> GDVVEAVENAVARVADTIGSGPSNSQAVPALTAVETGHTSQVTPSDTVQTRHVKNYHSRSESSIENFLSRSACVYMGEYHTTNSDQTKLFASWTISARRMVQMRRKLEIFTYVRFDVEVTFVITSKQDQGTQLGQDMPPLTHQIMYIPPGGPIPKSVTDYTWQTSTNPSIFWTEGNAPPRMSIPFISIGNAYSNFYDGWSHFSQNGVYGYNTLNHMGQIYVRHVNGSSPLPMTSTVRMYFKPKHVKAWVPRPPRLCQYKNASTVNFSPTDITDKRNSITYIPDTVKPDV;> SDRVRSITLGNSTITTQESANVVVGYGRWPEYLRDDEATAEDQPTQPDVATCRFYTLESVTWEKDSPGWWWKFPDALKDMGLFGQNMYYHYLGRAGYTIHVQCNASKFHQGCLLVVCVPEAEMGCSTVDGTVNEHGLSEGETAKKFSATGTNGTNTVQSIVTNAGMGVGVGNLTIFPHQWINLRTNNCATIVMPYINNVPMDNMFRHHNFTLMIIPFVPLNYSSDFSTYVPITVTVAPMCAEYNGLRLSTAL;> GLPVINTPGSNQFLTSDDFQSPSAMPQFDVTPELNIPGEVQNLMEIAEVDSVVPVNNVAGNLETMDIYRIPVQSGNHQSSQVFGFQVQPGLDGVFKHTLLGEILNYYAHWSGSIKLTFVFCGSAMATGKFLLAYAPPGANAPKSRK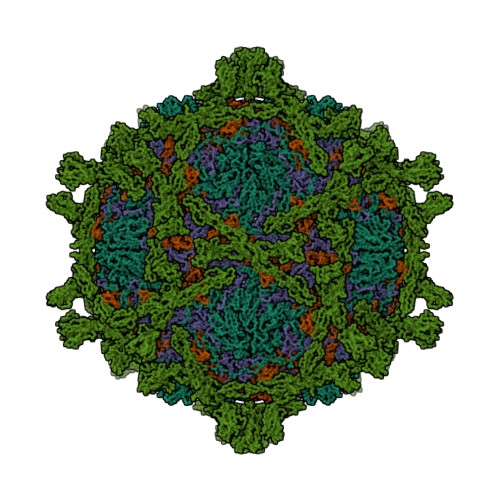DAMLGTHIIWDVGLQSSCVLCIPWISQTHYRLVQQDEYTSAGNVTCWYQTGIVVPAGTPTSCSIMCFVSACNDFSVRLLKDTPFIQQAALLQ;> GAQVSTQKTGAHESIIHYTNINYYKDAASNSANRQDFTQDPGKFTEPVKDIMVKSLPALN;> QDCGLPPDVPNAQPALEGRTSFPEDTVITYKCEESFVKIPGEKDSVICLKGSQWSDIEEFCNRSQDCGLPPDVPNAQPALEGRTSFPEDTVITYKCEESFVKIPGEKDSVICLKGSQWSDIEEFCNRSCEVPTRLNSASLKQPYITQNYFPVGTVVEYECRPGYRREPSLSPKLTCLQNLKWSTAVEFCKKKSCPNPGEIRNGQIDVPGGILFGATISFSCNTGYKLFGSTSSFCLISGSSVQWSDPLPECREIYCPAPPQIDNGIIQGERDHYGYRQSVTYACNKGFTMIGEHSIYCTVNNDEGEWSGPPPECRG> MASDKASSIELKFDRNKGEVGDILIGTVRINNIKNFAGFQVNIVYDPKVLMAVDPETGKEFTSSTFPPGRTVLKNNAYGPIQIADNDPEKGILNFALAYSYIAGYKETGVAEESGIIAKIGFKILQKKSTAVKFQD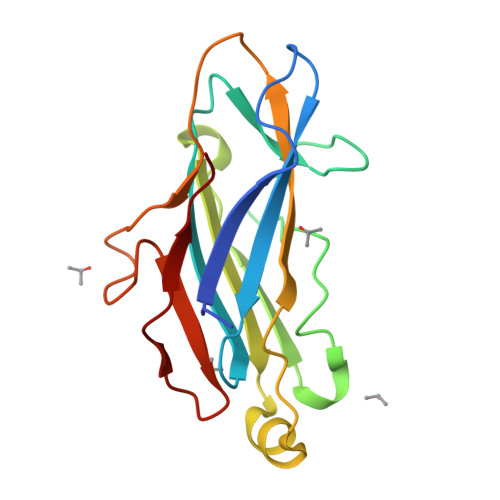TLSMPGAISGTQLFDWDGEVITGYEVIQPD>[4x]SRKTYTLTDYLKNTYRLKLYSLRWISDHEYLYKQENNILVFNAEYGNSSVFLENSTFDEFGHSINDYSISPDGQFILLEYNYVKQWRHSYTASYDIYDLNKRQLITEERIPNNTQWVTWSPVGHKLAYVWNNDIYVKIEPNLPSYRITWTGKEDIIYNGITDWVYEEEVFSAYSALWWSPNGT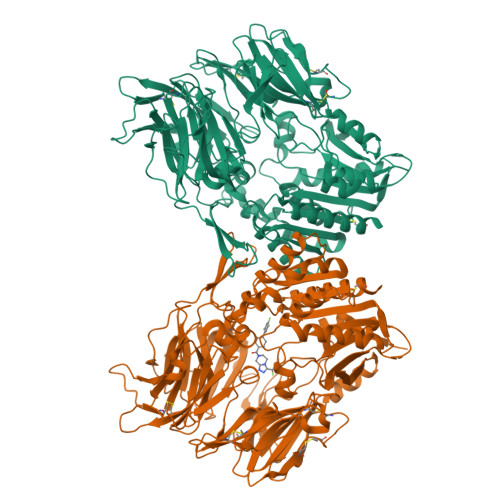FLAYAQFNDTEVPLIEYSFYSDESLQYPKTVRVPYPKAGAVNPTVKFFVVNTDSLSSVTNATSIQITAPASMLIGDHYLCDVTWATQERISLQWLRRIQNYSVMDICDYDESSGRWNCLVARQHIEMSTTGWVGRFRPSEPHFTLDGNSFYKIISNEEGYRHICYFQIDKKDCTFITKGTWEVIGIEALTSDYLYYISNEYKGMPGGRNLYKIQLSDYTKVTCLSCELNPERCQYYSVSFSKEAKYYQLRCSGPGLPLYTLHSSVNDKGLRVLEDNSALDKMLQNVQMPSKKLDFIILNETKFWYQMILPPHFDKSKKYPLLLDVYAGPCSQKADTVFRLNWATYLASTENIIVASFDGRGSGYQGDKIMHAINRRLGTFEVEDQIEAARQFSKMGFVDNKRIAIWGWSYGGYVTSMVLGSGSGVFKCGIAVAPVSRWEYYDSVYTERYMGLPTPEDNLDHYRNSTVMSRAENFKQVEYLLIHGTADDNVHFQQSAQISKALVDVGVDFQAMWYTDEDHGIASSTAHQHIYTHMSHFIKQCFS> MAKYTR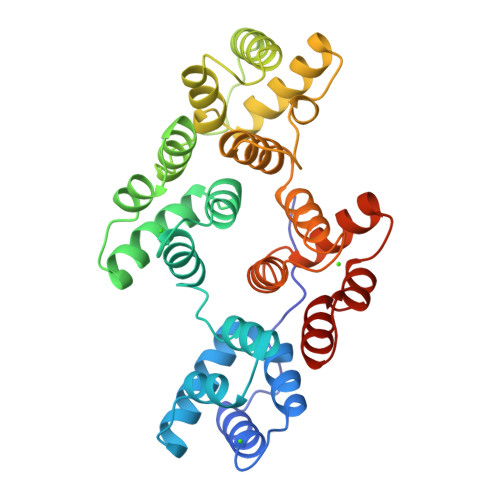GTVTAFSPFDARADAEALRKAMKGMGTDEETILKILTSRNNAQRQEIASAFKTLFGRDLVDDLKSELTGKFETLMVSLMRPARIFDAHALKHAIKGAGTNEKVLTEILASRTPAEVQNIKQVYMQEYEANLEDKITGETSGHFQRLLVVLLQANRDPDGRVEEALVEKDAQVLFRAGELKWGTDEETFITILGTRSVSHLRRVFDKYMTISGFQIEETIDRETSGDLEKLLLAVVKCIRSVPAYFAETLYYSMKGAGTDDDTLIRVMVSRSEIDLLDIRHEFRKNFAKSLYQMIQKDTSGDYRKALLLLCGGDDE> MAEKEEAIFRSAEMALVQFYIPQEISRDSAYTLGQLGLVQFRDLNSKVRAFQRTFVNEIRRLDNVERQYRYFYSLLKKHDIKLYEGDTDKYLDGSGELYVPPSGSVIDDYVRNASYLEERLIQMEDATDQIEVQKNDLEQYRFILQSGDEFFLKGDNTDSTSYMDEDMIDANGENIAAAIGASVNYVTGVIARDKVATLEQILWRVLRGNLFFKTVEIEQPVYDVKTREYKHKNAFIVFSHGDLIIKRIRKIAESLDANLYDVDSSNEGRSQQLAKVNKNLSDLYTVLKTTSTTLESELYAIAKELDSWFQDVTREKAIFEILNKSNYDTNRKILIAEGWIPRDELATLQARLGEMIARLGIDVPSIIQVLDTNHTPPTFHRTNKFTAGFQSICDCYGIAQYREINAGLPTIVTFPFMFAIMFGDMGHGFLMTLAALSLVLNEKKINKMKRGEIFDMAFTGRYIILLMGVFSMYTGFLYNDIFSKTMTIFKSGWKWPDHWKKGESITATSVGTYPIGLDWAWHGTENALLFSNSYKMKLSILMGFIHMTYSYFFSLANHLYFNSMIDIIGNFIPGLLFMQGIFGYLSVCIVYKWAVDWVKDGKPAPGLLNMLINMFLSPGTIDDELYPHQAKVQVFLLLMALVCIPWLLLVKPLHFKFTHKKKSHEPLPSTEADASSEDLEAQQLISAMDADDAEEEEVGSGSHGEDFGDIMIHQVIHTIEFCLNCVSHTASYLRLWALSLAHAQLSSVLWTMTIQIAFGFRGFVGVFMTVALFAMWFALTCAVLVLMEGTSAMLHSLRLHWVESMSKFFVGE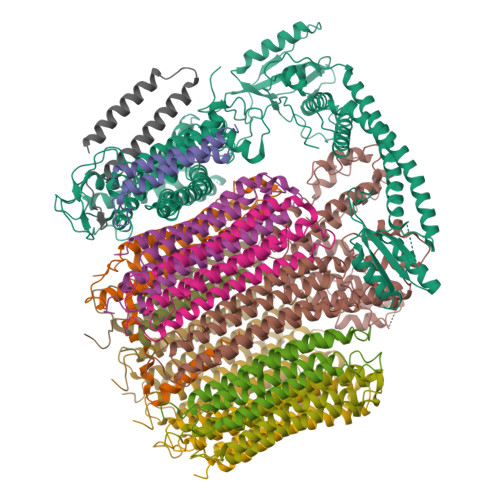GLPYEPFAFEYKDMEVAVASASSSASSDYKDHDGDYKDHDIDYKDDDDK;> MVFGQLYALFIFTLSCCISKTVQADSSKESSSFISFDKESNWDTISTISSTADVISSVDSAIAVFEFDNFSLLDNLMIDEEYPFFNRFFANDVSLTVHDDSPLNISQSLSPIMEQFTVDELPESASDLLYEYSLDDKSIVLFKFTSDAYDLKKLDEFIDSCLSFLEDKSGDNLTVVINSLGWAFEDEDGDDEYATEETLSHHDNNKGKEGDDDILSSIWTEGLLMCLIVSALLLFILIVALSWISNLDITYGALEKSTNPIKKNN;> MNKESKDDDMSLGKFSFSHFLYYLVLIVVIVYGLYKLFTGHGSDINFGKFLLRTSPYMWANLGIALCVGLSVVGAAWGIFITGSSMIGAGVRAPRITTKNLISIIFCEVVAIYGLIIAIVFSSKLTVATAENMYSKSNLYTGYSLFWAGITVGASNLICGIAVGITGATAAISDAADSALFVKILVIEIFGSILGLLGLIVGLLMAGKASEFQ;> MEGVYFNIDNGFIEGVVRGYRNGLLSNNQYINLTQCDTLEDLKLQLSSTDYGNFLSSVSSESLTTSLIQEYASSKLYHEFNYIRDQSSGSTRKFMDYITYGYMIDNVALMITGTIHDRDKGEILQRCHPLGWFDTLPTLSVATDLESLYETVLVDTPLAPYFKNCFDTAEELDDMNIEIIRNKLYKAYLEDFYNFVTEEIPEPAKECMQTLLGFEADRRSINIALNSLQSSDIDPDLKSDLLPNIGKLYPLATFHLAQAQDFEGVRAALANVYEYRGFLETGNLEDHFYQLEMELCRDAFTQQFAISTVWAWMKSKEQEVRNITWIAECIAQNQRERINNYISVY;> MSSFYTVVGVFIVVSAMSVLFWIMAPKNNQAVWRSTVILTLAMMFLMWAITFLCQLHPLVAPRRSDLRPEFAE;> MRPVVSTGKAWCCTVLSAFGVVILSVIAHLFNTNHESFVGSINDPEDGPAVAHTVYLAALVYLVFFVFCGFQVYLARRKPSIELR;>[8x]MTELCPVYAPFFGAIGCASAIIFTSLGAAYGTAKSGVGICATCVLRPDLLFKNIVPVIMAGIIAIYGLVVSVLVCYSLGQKQALYTGFIQLGAGLSVGLSGLAAGFAIGIVGDAGVRGSSQQPRLFVGMILILIFAEVLGLYGLIVALLLNSRATQDVVC;> MSTQLASNIYAPLYAPFFGFAGCAAAMVLSCLGAAIGTAKSGIGIAGIGTFKPELIMKSLIPVVMSGILAIYGLVVAVLIAGNLSPTEDYTLFNGFMHLSCGLCVGFACLSSGYAIGMVGDVGVRKYMHQPRLFVGIVLILIFSEVLGLYGMIVALILNTRGSE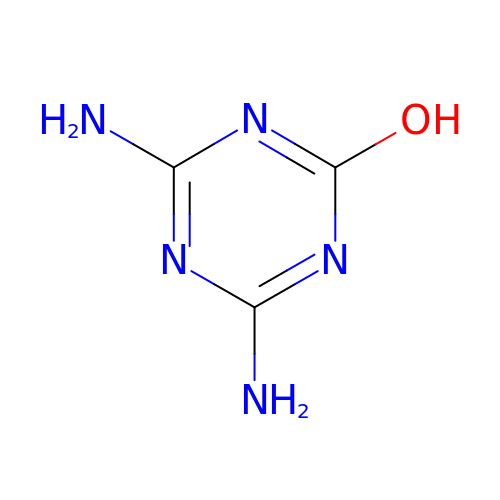4,6-diamino-1,3,5-triazin-2-ol | C3 H5 N5 O | MASBWURJQFFLOO-UHFFFAOYSA-N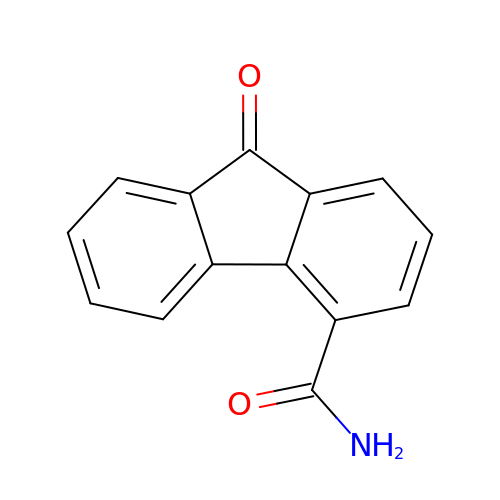9-oxo-9H-fluorene-4-carboxamide | C14 H9 N O2 | PRROCNFTWSJBTJ-UHFFFAOYSA-N> MTATADAAETGNGHITGFGSKPYRSYVLLALTLIYTLNFIDRTVITVVAQPIINTFSLSDAQWGLLTGPPFALFYALMGIPIAMWADRGNRVFIISLCVIIWSIMTVFCG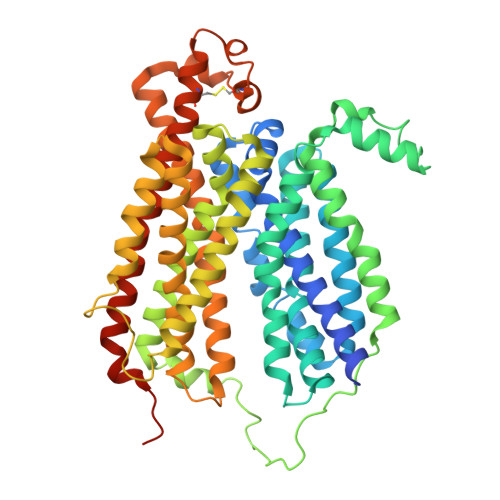LAASFIWLLLFRVGVAIGEAGCTPPANSIITDYYPPKSRANAIGIYSMGVTVGGVMAQLFGGALAGLQGADFGNFLSSIGLGWLFSGINWEEVEGWRLVFVIVGAPGILVALILWLTTREPPRGYSDPKGKTPLEKAGFFEAFREFGAKPTFWSLSLGAAFVAFVGYGLISFQAPFLMRVHGVSVSEAAIRYGAPLAAVAAFGTFLGGFLSEKFTPRFPAIVAWLPGVGLLIAIPAYIAAFLTPSLTMAFWMWVIAAIAHYAYLGAQYTVSTAIVSPRSRATTVSVLLLIVSLIGNGLGPMFTGMMSSAFMGGIIRKNGLEEAFATFNPGLCAGRMAEIGEMGPALCSAYAEGLRQSMVATVVFLVIAAAFYFLASRTFLKDRWSPAADAAAENLYFQ> GMAQEKSALSKAQKAAVLLLSLPEEVSMNIVKELSEEELQKLFALAKDLESVPEEEIENIA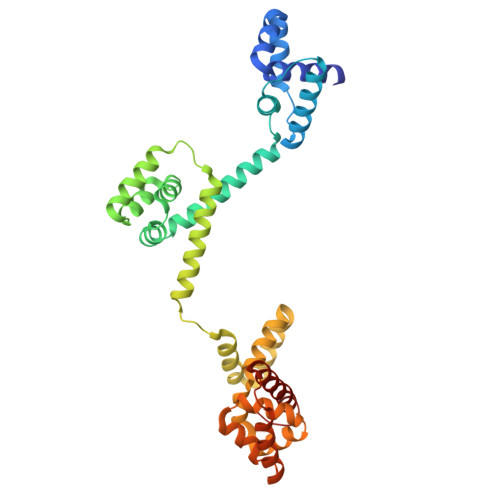EELLDEIKKAGIKIKKPEEFIENIKKVIPPTLAEKFRGILELGDAEKILKEIEKVDSRILASLLKNEHPQTIALFLSQLSPKKSAEIIQNLPEELKKEVVKRIATLENVNVQYVKELAQILLEEISSLGAKEALKLEGTAVAAELLNTLDKETRELILQSIGQEDPLLEERIREKMFTFEDIRKLSDRDIIEILKVVDKNTLMIALLGAPEDIKQKFLSNMSKRAAKLFLEDMEALGPVKKSEIEKAQRQVVNIIRKMIDEGKIEIGD>MAKDIGINSDPNSSSVDKLMKSSGVSNPTYTLVWKVWILAVTLYYAIRIPLTLVFPSLFSPLLPLDILASLALIADIPLDLAFESRRTSGRKPTLLAPSRLPDLLAALPLDLLVFALHLPSPLSLLSLVRLLKLISVQASATRILSYRINPALLRLLSLVGFILLAAHGIACGWMSLQPPSENPAGTRYLSAFYWTITTLTTIGYGDITPSTPTQTVYTIVIELLGAAMYGLVIGNIASLVSKLDAAKLLHRERVERVTAFLSYKRISPELQRRIIEYFDY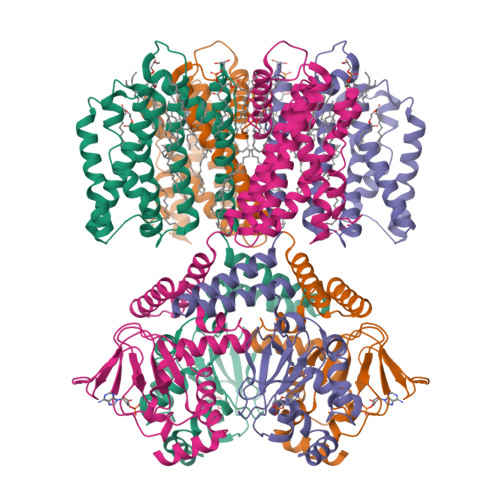LWETRRGYEEREVLKELPHPLRLAVAMEIHGDVIEKVPLFKGAGEEFIRDIILHLEPVIYGPGEYIIRAGEMGSDVYFINRGSVEVLSADEKTRYAILSEGQFFGEMALILRAPRTATVRARAFCDLYRLDKETFDRILSRYPEIAAQIQELAVRRKELESSGLVPRGSVKHHHH[4x]>[2x]GIDPFTTRPSSDLTAFREHFAKAKHIAIITGAGVSAESGVPTFRGPGGFWRKWQAQDLATPEAFSRDPSLVWEFYHYRREVMRSKMPNPAHLAIAECEARLGQQGRSVVIITQNIDELHHRAGSKHVYEIHGSLFKTRCMSCGEVKANHKSPICPALDGKGAPDPNTKEARIPVELLPRCERKSCNGLLRPHVVWFGETLDSDILTAVERELEKCDLCLVVGTSSIVYPAAMFAPQVASRGVPVAEFNMECTPATQRFKYHFEGPCGSTLPPALE;> XVLKEYGV

Among the protein Lys deacetylases, sirtuins form the evolutionary defined class III. Sirtuins are increasingly recognized as deacylases with isoform-specific acyl selectivities, catalyzing removal of acylations emerging as posttranslational protein modifications, such as succinylation or crotonylation. The sirtuin core comprises a Rossmann-fold subdomain and a smaller Zn2+-binding module. The isoform differences in preferred substrate acyls are caused by binding of the acyl moiety to an active site channel with isoform-specific features.

Attempts to solve a Sirt4 structure in complex with substrate peptide to study acyl recognition details failed, possibly due to the lacking stabilization by this ligand, but we were able to solve a complex of zebrafish Sirt5 (zSirt5) with HMG-CPS1 peptide. The HMG length is reduced through a helical conformation, albeit with opposite handedness compared to glutaryl-CPS1, to position the 3-hydroxy and 3-methyl moieties toward Ile138/His154 and Tyr98/Val216, respectively. The distal carboxylate interacts with Tyr98 and Arg101, which also recognize the carboxylates of succinyl and glutaryl substrates. Interestingly, Sirt4 also features such a Tyr-X-X-Arg motif in α5. The Sirt4 motif is shifted one helix turn, however, with Sirt4-Tyr104 oriented back to the region occupied by Sirt5-Tyr98, but Sirt4-Arg107 pointing away from the acyl channel. Sirt4 residues in the positions of Sirt5-Tyr98/Arg101 would be Asn108 and Gly111. Due to a slightly different conformation, however, Gly111 is shifted and the area of Sirt5-Arg101 is occupied by the Sirt4-loop residue Asp201, which would result in close contacts between the carboxylates of Asp201 and an HMG substrate. Sirt5 activity against HMG-CPS1 thus exceeds that of Sirt4 mainly due to faster turnover, and this Sirt5 activity appears even higher with other peptide sequences, but it is still 60–80% lower than the enzyme’s desuccinylase activity.[(1R)-1-amino-2-phenylethyl]phosphonic acid | C8 H12 N O3 P | 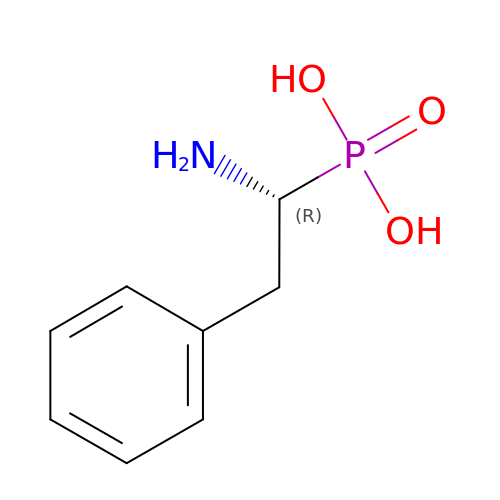FQCNOURLMNHAQN-MRVPVSSYSA-N>[2x]AAVILESIFLKRSQQKKKTSPLNFKKCLFLLTVHKLSYYEYDFERGRRGSKKGSIDVEKITCVETVVPEKNPPPERQIPRRGEESSEMEQISIIERFPYPFQVVYDEGP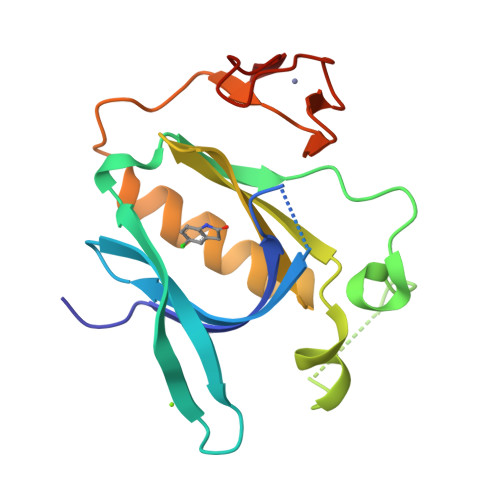LYVFSPTEELRKRWIHQLKNVIRYNSDLVQKYHPCFWIDGQYLCCSQTAKNAMGCQILEN>[2x]SMDNLVLIRMKPDENGRFGFNVKGGYDQKMPVIVSRVAPGTPADLCV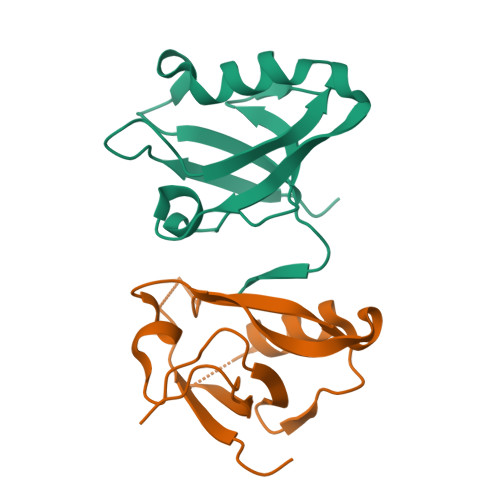PRLNEGDQVVLINGRDIAEHTHDQVVLFIKASCERHSGELMLLVRPNAVESTV> MSTKQHSAKDELLYLNKAVVFGSGAFGTALAMVLSKKCREVCVWHMNEEEVRLVNEKRENVLFLKGVQLASNITFTSDVEKAYNGAEIILFVIPTQFLRGFFEKSGGNLIAYAKEKQVPVLVCTKGIERSTLKFPAEIIGEFLPSPLLSVLAGPSFAIEVATGVFTCVSIASADINVARRLQRIMSTGDRSFVCWATTDTVGCEVASAVKNVLAIGSGVANGLGMGLNARAALIMRGLLE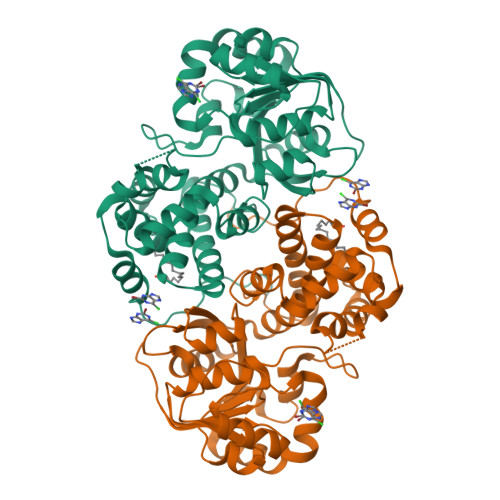IRDLTAALGGDGSAVFGLAGLGDLQLTCSSELSRNFTVGKKLGKGLPIEEIQRTSKAVAEGVATADPLMRLAKQLKVKMPLCHQIYEIVYKKKNPRDALADLLSCGLQDEGLPPLFKRSASTPSKL> MLPLYLLTNAKGQQMQIELKNGEIIQGILTNVDNWMNLTLSNVTEYSEESAINSEDNAESSKAVKLNEIYIRGTFIKFI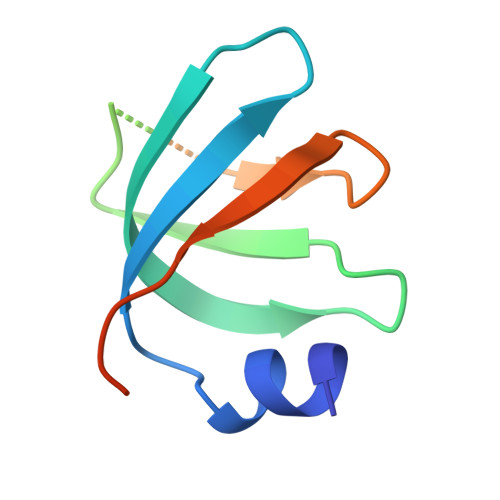KLQDNIIDKVKQQI[(2~{R},3~{S},4~{R},5~{R})-5-(6-aminopurin-9-yl)-3,4-bis(oxidanyl)oxolan-2-yl]methyl ~{N}-(3-chloranyl-2-methyl-phenyl)carbonylsulfamate | C18 H19 Cl N6 O7 S | 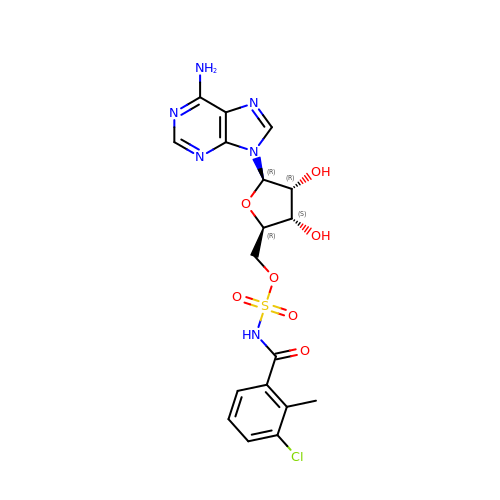NHHJUHWTWOXCDU-XWXWGSFUSA-N>MPTLVNGPRRDSTEGFDTDIITLPRFIIEHQKQFKNATGDFTLVLNALQFAFKFVSHTIRRAELVNLVGLAGASNFTGDQQKKLDVLGDEIFINAMRASGIIKVLVSEEQEDLIVFPTNTGSYAVCCDPIDGSSNLDAGVSVGTIASIFRLLPDSSGTINDVLRCGKEMVAACYAMYGSSTHLVLTLGDGVDGFTLDTNLGEFILTHPNLRIPPQKAIYSINEGNTLYWNETIRTFIEKVKQPQADNNNKPFSARYVGSMVADVHRTFLYGGLFAYPCDKKSPNGKLRLLYEAFPMAFLME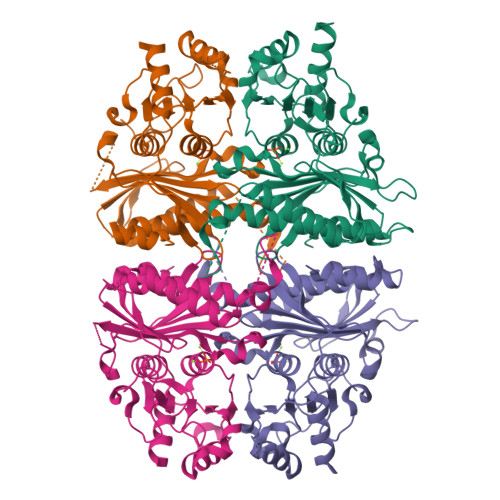QAGGKAVNDRGERILDLVPSHIHDKSSIWLGSSGEIDKFLDHIGKSQHHHHHH[4x]> DW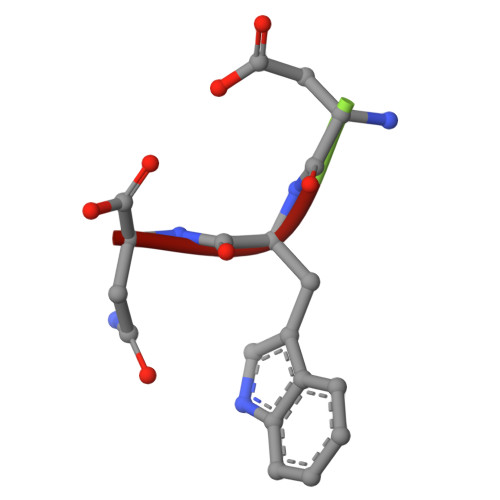N3-pyridin-2-ylbenzoic acid | C12 H9 N O2 | 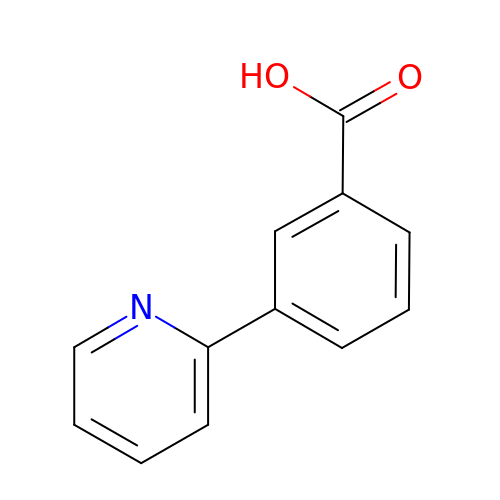IRXFQXMHMRTLIR-UHFFFAOYSA-N>TVAYIAIGSNLASPLEQVNAALKALGDIPESHILTVSSFYRTPPLGPQDQPDYLNAAVALETSLAPEELLNHTQRIELQQGRVRKAERAGPRTLDLDIMLFGNEVINTERLTVPHYDMKNRGFMLWPLFEIAPELVFPDGEMLRQILHTRAFDKL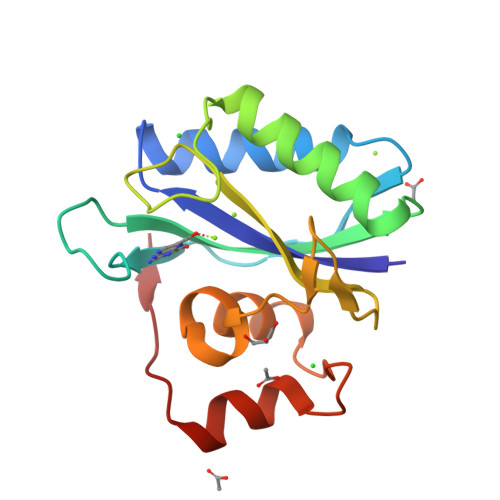NKW[2x]> MNEQYSALRSNVSMLGKVLGETIKDALGEHILERVETIRKLSKSSRAGNDANRQELLTTLQNLSNDELLPVARAFSQFLNLANTAEQYHSISPKGEAASNPEVIARTLRKLKNQPELSEDTIKKAVESLSLELVLTAHPTEITRRTLIHKMVEVNACLKQLDNKDIADYEHNQLMRRLRQLIAQSWHTDEIRKLRPSPVDEAKWGFAVVENSLWQGVPNYLRELNEQLEENLGYKLPVEFVPVRFTSWMGGDRDGNPNVTADITRHVLLLSRWKATDLFLKDIQVLVSELSMVEATPELLALVGEEGAAEPYRYLMKNLRSRLMATQAWLEARLKGEELPKPEGLLTQNEELWEPLYACYQSLQACGMGIIANGDLLDTLRRVKCFGVPLVRIDIRQESTRHTEALGELTRYLGIGDYESWSEADKQAFLIRELNSKRPLLPRNWQPSAETREVLDTCQVIAEAPQGSIAAYVISMAKTPSDVLAVHLLLKEAGIGFAMPVAPLFETLDDLNNANDVMTQLLNIDWYRGLIQGKQMVMIGYSDSAKDAGVMAASWAQYQAQDALIKTCEKAGIELTLFHGRGGSIGRGGAPAHAALLSQPPGSLKGGLRVTEQGEMIRFKYGLPEITVSSLSLYTGAILEANLLPPPEPKESWRRIMDELSVISCDVYRGYVRENKDFVPYFRSATPEQELGKLPLGSRP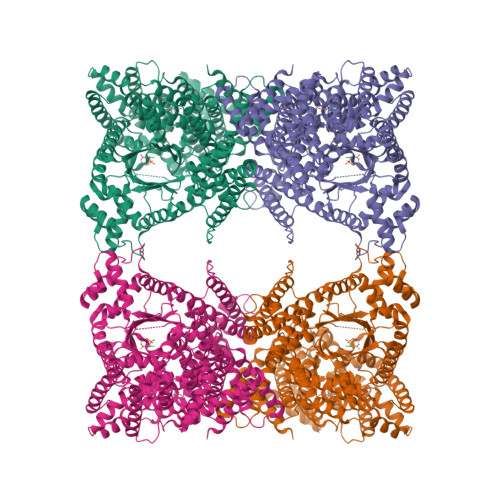AKRRPTGGVESLRAIPWIFAWTQNRLMLPAWLGAGTALQKVVEDGKQSELEAMCRDWPFFSTRLGMLEMVFAKADLWLAEYYDQRLVDKALWPLGKELRNLQEEDIKVVLAIANDSHLMADLPWIAESIQLRNIYTDPLNVLQAELLHRSRQAEKEGQEPDPRVEQALMVTIAGIAAGMRNTG>ESSTQLDIVIVLDGSNSIYPWDSVTAFLNDLLERMDIGPKQTQVGIVQYGENVTHEFNLNKYSSTEEVLVAAKKIVQRGGRQTMTALGTDTARKEAFTEARGARRGVKKVMVIVTDGESHDNHRLKKVIQDCEDENIQRFSIAILGSYNRGNLSTEKFVEEIKSIASEPTEKHFFNVSDALALVTIVKTLGERIFALEATA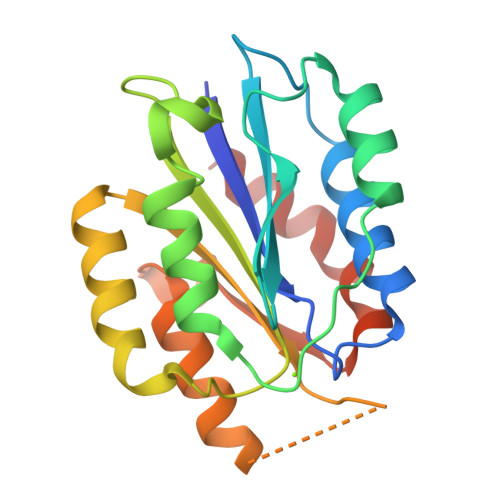[2x]> RITRLQE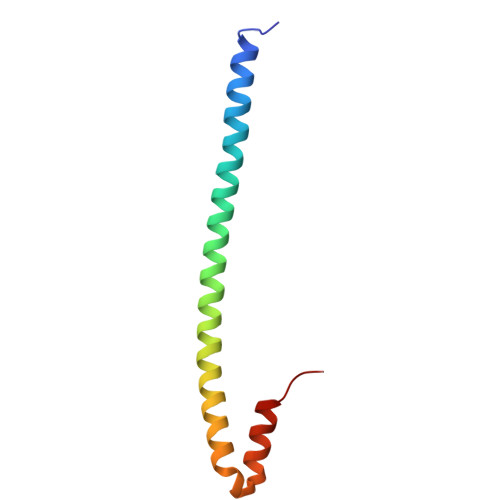KEDLQELNDRLAVYIDRVRSLETENAGLRLRITESEEVVDFYFGKLRNIELICQENEGENDPVLQRIVDILYATDE>[2x]GSHMDSTTIQQNKDTLSQIVVF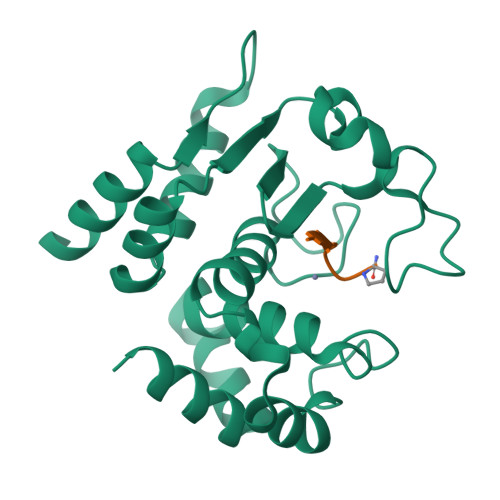PTGNYDKNEANAMVNRLANIDGKYLNALKQNNLKIKLLSGKLTDEKEYAYLKGVVPKGFEGTGKTWDDVPGLGGSTVALRIGFSNKGKGHDAINLELHATAHAIDHIVLNDISKSAQFKQIFAKEGRSLGNVNFLGVYPEEFFAESFAYYYLNQDTNSKLKSACPQTYSFLQNLAK;>[2x]XEVNPPVP>LSECKTGNGKNYRGTMSKTKNGITCQKWSSTSPHRPRFSPATHPSEGLEENYCRNPDNDPQGPWCYTTDPEKRYDYCD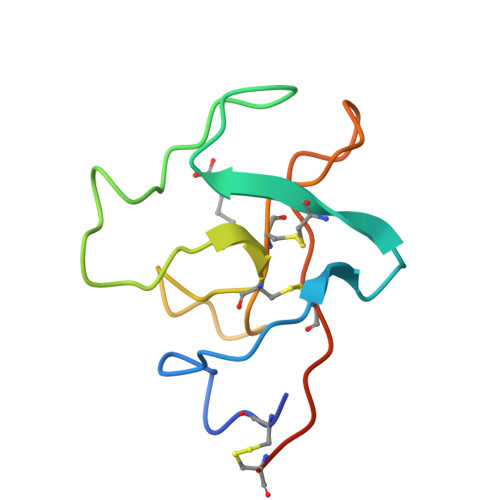ILECEEECMH[2x]5-[2-CHLORO-4-(TRIFLUOROMETHYL)PHENOXY]-2-NITROBENZOIC ACID | C14 H7 Cl F3 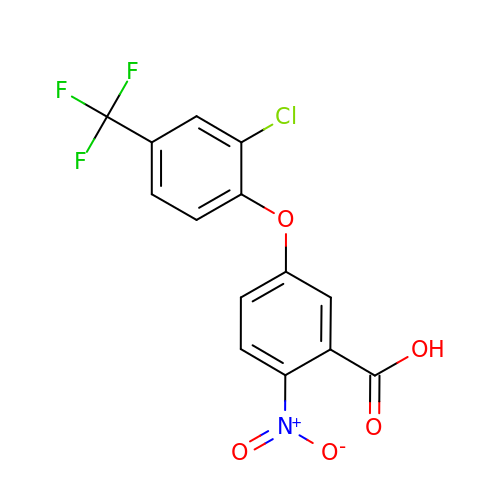N O5 | NUFNQYOELLVIPL-UHFFFAOYSA-N>MDLEKNYPTPRTSRTGHGGVNQLGGVFVNGRPLPDVVRQRIVELAHQGVRPCDISRQLRVSHGCVSKILGRYYETGSIKPGVIGGSKPKVATPKVVEKIAEYKRQNPTMFAWEIRD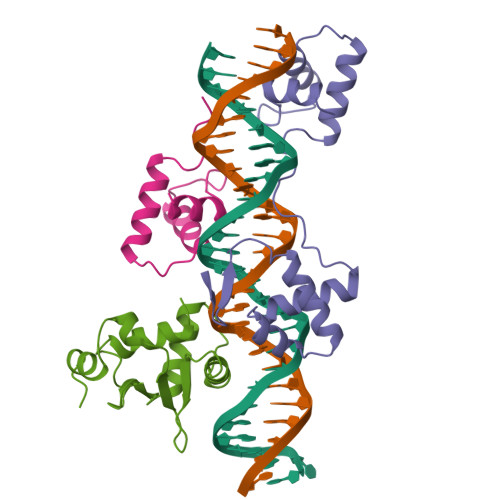RLLAERVCDNDTVPSVSSINRIIRTKVQQPPNQ[3x];>GSGPIQLWQFLLELLTDKSCQSFISWTGDGWEFKLSDPDEVARRWGKRKNKPKMNYEKLSRGLRYYYDKNIIHKTAGKRYVYRFVCDLQSLLGYTPEELHAMLDVKPDAD[2x]In this work, we exhaustively probe the ability of all 36 immobile HJ sequences to form DNA crystals in two different designed systems. Three separate self-assembling DNA crystal systems are described in this report: the “4 × 5” and “4 × 6” designs (collectively referred to as the 4 × N systems), and a third construct with a “scrambled” sequence variant of the 4 × 6 lattices. Self-assembly was mediated by three constituent oligonucleotides: (S1) containing four sequence repeats of either 5 or 6 bases; (S2) composed of 21 bases containing complementary regions to both (S1); and (S3) which forms the second junction crossover. The HJ serves as the fundamental component at the core of each unit, and the ultimate assembly of the full lattice is facilitated by the complementary 2-base sticky ends that tail each duplex.

Each asymmetric unit could be defined as either a HJ containing 10 and 11 bp on each arm, or as a 21-bp linear duplex. To investigate this possibility, we designed “scrambled” sequences with targeted base substitutions, while maintaining GC content, along each “stem”. Contrary to the buffer preference observed with the native P32 crystals, the scrambled systems exhibited an exclusive preference towards low salt buffers, much like the native R3 crystals. Remarkably, only J1 and J2 retained the P32 symmetry, with all others yielding an R3 lattice. There appeared to be only a marginal difference in the average cell lengths in the R3 scramble crystals (a = b = 113.04 c = 51.10) relative to the native 4 × 6 sequences: the a, b axis trended ~2 Å shorter and c ~1.3 Å longer, whereas in the J1 and J2 cases, the crystals were in good agreement with the original 4 × 6 motif. The average angles of the R3 and P32 crystals were 61.00° (σ = 1.21) and 58.05° (σ = 1.39), respectively. However, in the majority of the crystal structures reported here, the cacodylate anion indeed fits best into the electron density map of our X-ray structures, due to the presence of sodium cacodylate in the crystallization solution.

> ACGTCT;> GAACGACAGAGACGTCGACTC;> TCGAGTCG;> CTGTCGT3-{[(4-CARBOXY-2-HYDROXYANILINE]SULFONYL}THIOPHENE-2-CARBOXYLIC ACID | C12 H9 N O7 S2 | 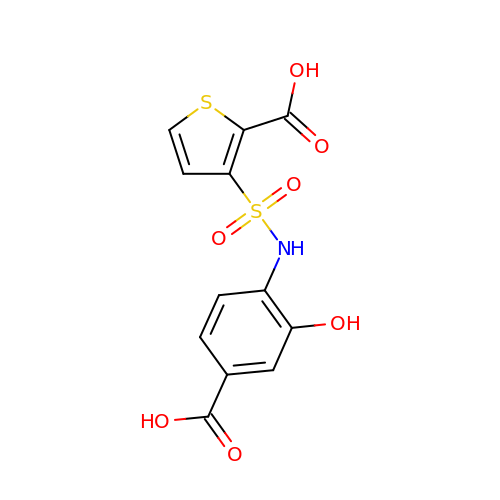RDPXXOOKKRIKFN-UHFFFAOYSA-N>SATTPPGDLEQPELEARVKEIIEVDGYQFRDLNDNGELDPYEDWRLPTPERVADLVGQMSLVEKSGLMLINTLNAACDPQTGEFGVLPAQADNYINTQHMHRFVFRNVVDVRAEGVECTGTGTPVVSPAEAATFTNAVQEMSEATRLGIPSLFKSNARNHIDPDARVGINEAAGAFSAFPKEAGIAAAALGEQARRTGEATTGDMSVVADFADVMGEEWASIGLRGMYGYMADLSTEPRWYRTHETFTEDAYLAAEIMETLVQTLQGEELTDNGLALSPQTRVALTLKHFPGGGPQELGLDPHYAFGKAQVYPAGRFEEHFLPFQAAIDAGVSSIMPYYGVPVDVPVVGGEPGETYPHTGFAFSDSIVNGLLRDQLGFTGYVNSNTGIINDRAWGLEGNTVPERVAAAINGGTDTLSGFSDVSVITDLYEADLISEERIDLAAERLLEPLFDMGLFENPYVDPDVATATVGADDHRAVGLDLQRKSLVLLQNEETDEGPVLPLKEGGDVYILGDFTEETVESYGYEVTNGNVAEGEERPSAAGSDYVLISMTAKTNAGDYVSDDP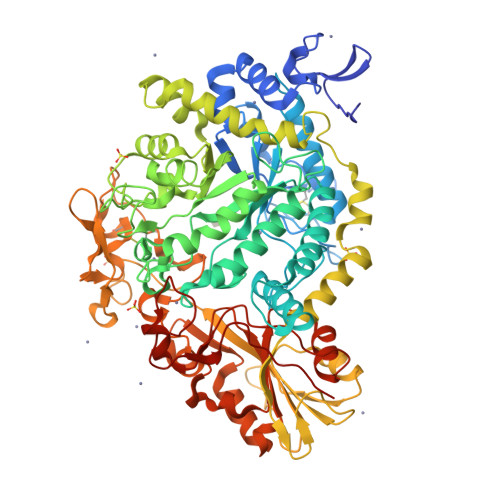SLGLNPDHGTNPSVIIGDDGEPLPGLDGQSLWGAADVCVHKEGHEENPSCTDNRLRFGGAYPWESSILDFTGMEAAESWEVVPSLETIQEVMAEVEDPSKVILHVYFRQPYVLDEESGLRDAGAILAGFGMTDTALMDVLTGAYAPQGKLPFALAGTREAIIEQDSDRPGYDETEDGALYPFGYGLTYEDDTEE[2x]>PPYTVVYFPVRGRCAALRMLLADQGQSWKEE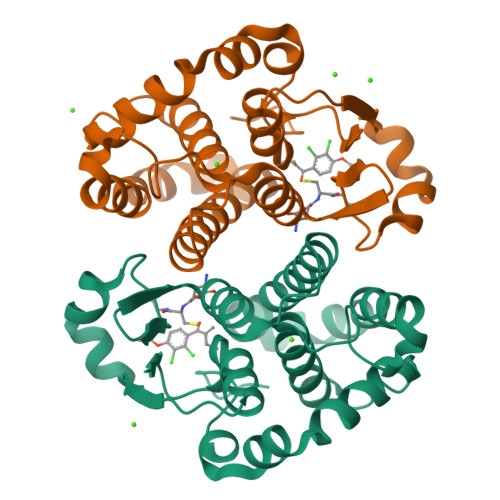VVTVETWQEGSLKASSLYGQLPKFQDGDLTLYQSNTILRHLGRTLGLYGKDQQEAALVDMVNDGVEDLRCKYISLIVTNYEAGKDDYVKALPGQLKPFETLLSQNQGGKTFIVGDQISFADYNLLDLLLIHEVLAPGCLDAFPLLSAYVGRLSARPKLKAFLASPEYVNLPINGNGKQ[2x]> MERYENLFAQLNDRREGAFVPFVTLGDPGIEQSLKIIDTLIDAGADALELGVPFSDPLADGPTIQNANLRAFAAGVTPAQCFEMLALIREKHPTIPIGLLMYANLVFNNGIDAFYARCEQVGVDSVLVADVPVEESAPFRQAALRHNIAPIFICPPNADDDLLRQVASYGRGYTYLLSRSGVTGAENRGALPLHHLIEKLKEYHAAPALQGFGISSPEQVSAAVRAGAAGAISGSAIVKIIEKNLASPKQMLAELRSFVSAMKAASRA;> TTLLNPYFGEFGGMYVPQILMPALNQLEEAFVSAQKDPEFQAQFADLLKNYAGRPTALTKCQNITAGTRTTLYLKREDLLHGGAHKTNQVLGQALLAKRMGKSEIIAETGAGQHGVASALASALLGLKCRIYMGAKDVERQSPNVFRMRLMGAEVIPVHSGSATLKDLWNEALRDWSGSYETAHYMLGTAAGPHPYPTIVREFQRMIGEETKAQILDKEGRLPDAVIACVGGGSNAIGMFADFINDTSVGLIGVEPGGHGIETGEHGAPLKHGRVGIYFGMKAPMMQTADGQIEESYSISAGLDFPSVGPQHAYLNSIGRADYVSITDDEALEAFKTLCRHEG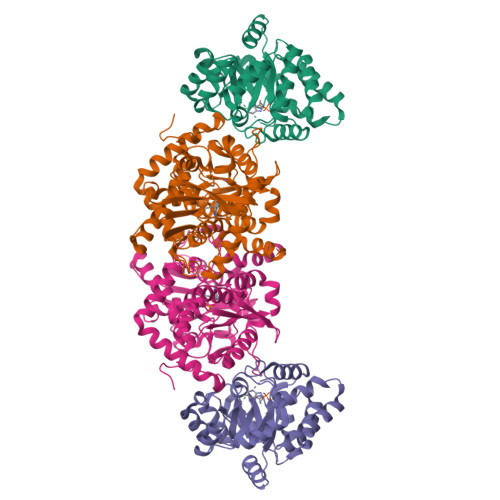IIPALESSHALAHALKMMREQPEKEQLLVVNLSGRGDKDIFTVHDILKARGEI> MDDLTIEILTDDADYDLQRFDCGEEALNLFLTTHLVRQHRNKILRA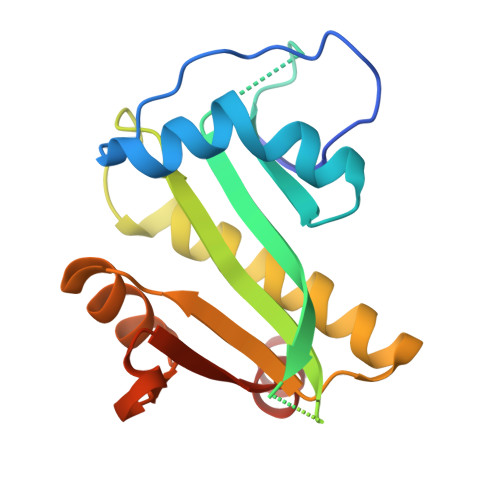YILCRNTPERQVLGYYTLCGSCFERAALPSKSKQKKIPYKNIPSVTLGRLAIDRSLQGQGWGATLVAHAMKVVWSASLAVGIHGLFVEALNEKAHTFYKSLGFIPLVGENENALFFPTKSIELLFTQSD> FMVSLPRMVYPQPKVLTPCRKDVLVVTPWLAPIVWEGTFNIDILNEQFRLQNTTIGLTVFAIKKYVAFLKLFLETAEKHFMVGHRVHYYVFTDQPAAVPRVTLGTGRQLSVLEVGAYKRWQDVSMRRMEMISDFCERRFLSEVDYLVCVDVDMEFRDHVGVEILTPL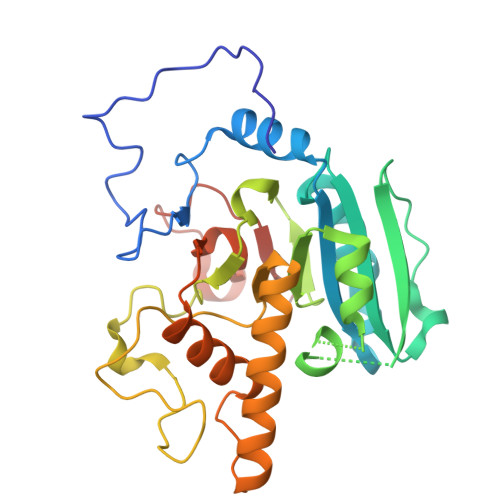FGTLHPSFYGSSREAFTYERRPQSQAYIPKDEGDFYYMGAFFGGSVQEVQRLTRACHQAMMVDQANGIEAVWHDCSHLNKYLLRHKPTKVLSPEYLWDQQLLGWPAVLRKLRFTAVPKNHQAVRNPE>MTIMAPEAVGESLDPRDPLLRLSNFFDDGSVELLHERDRSGVLAAAGTVNGVRTIAFCT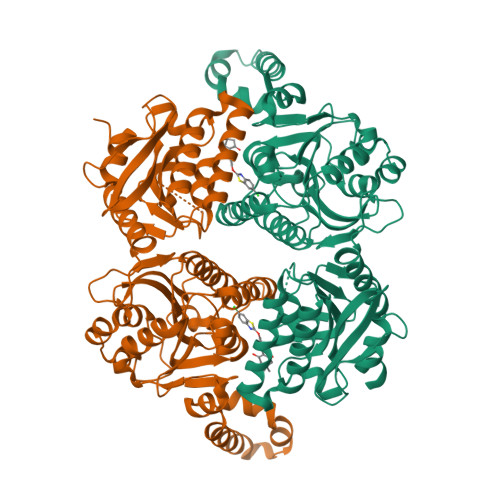DGTVMGGAMGVEGCTHIVNAYDTAIEDQSPIVGIWHSGGARLAEGVRALHAVGQVFEAMIRASGYIPQISVVVGFAAGGAAYGPALTDVVVMAPESRVFVTGPDVVRSVTGEDVDMASLGGPETHHKKSGVCHIVADDELDAYDRGRRLVGLFCQQGHFDRSKAEAGDTDIHALLPESSRRAYDVRPIVTAILDADTPFDEFQANWAPSMVVGLGRLSGRTVGVLANNPLRLGGCLNSESAEKAARFVRLCDAFGIPLVVVVDVPGYLPGVDQEWGGVVRRGAKLLHAFGECTVPRVTLVTRKTYGGAYIAMNSRSLNATKVFAWPDAEVAVMGAKAAVGILHKKKLAAAPEHEREALHDQLAAEHERIAGGVDSALDIGVVDEKIDPAHTRSKLTEALAQAPARRGRHKNIPL[8x]> MKTTLLKTLTPELHLVQHNDIPVLHLKHAVGTAKISLQGAQLISWKPQNAKQDVLWLSEVEPFKNGNAIRGGVPICYPWFGGVKQPAHGTARIRLWQLSHYYISVHKVRLEFELFSDLNIIEAKVSMVFTDKCHLTFTHYGEESAQAALHTYFNIGDINQVEVQGLPETCFNSLNQQQENVPSPRHISENVDCIYSAENMQNQILDKSFNRTIALHHHN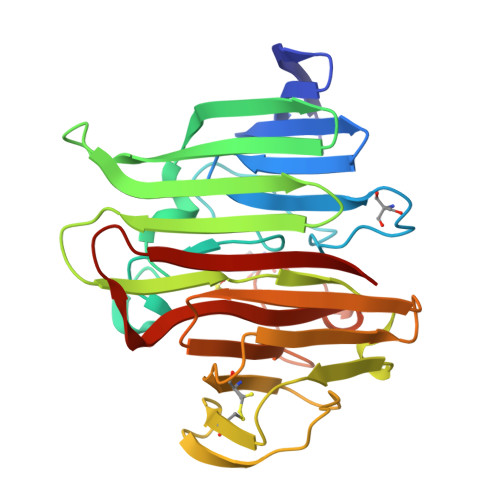ASQFVLWNPWHKKTSGMSETGYQKMLCLETARIHHLLEFGESLSVEISLKG4-(dibenzo[1,2-a:2',1'-d][7]annulen-11-ylidene)-1-methyl-piperidine 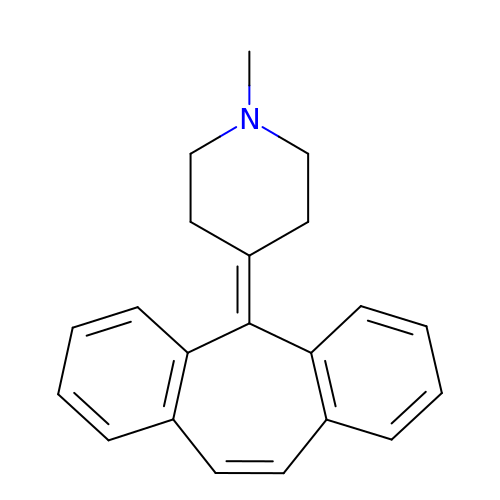| C21 H21 N | JJCFRYNCJDLXIK-UHFFFAOYSA-N> NLFDDNIDIFAD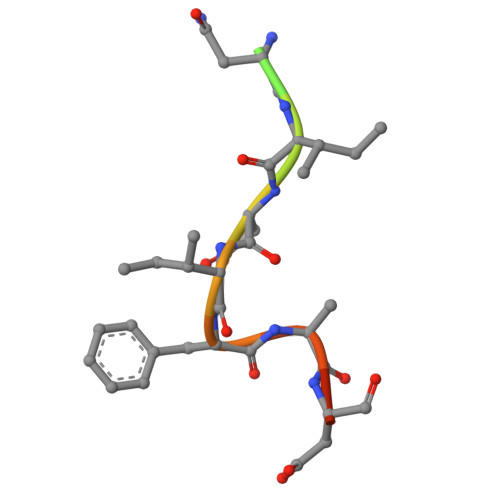LT>[8x]LEQKLISEEDLRSDKFRIMVQFLQANQESFMNGICGIMALASAQMYSSFEFTCPCLPDYNYA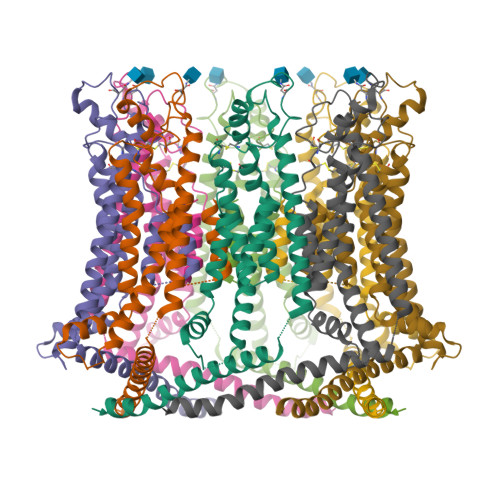YGIGILIVPPIWFFLLGYVMNNNISVLTEEWKRPVGKRSKDPAVLRYMFSSMTQRALIAPAVWIAVTLMDGKSFLCAFSPTADLSEFVNESYQSLSQKELLKIQAKIPCKDIFEEHEIISREAATRYIRCLSQACGWTFLMVITLVAFLVRAIRPCFTQAAFLKTKYWSHYIDTERKLFDETCKEHAKSFAKVCIQQYFESISGEIVSQLPQSPAKKGKGNKDEDGEKQKSDEERLLGIRKEGDMNKVLWNWHTCKPPLLLSKRTEEMNGHAHLDTHSLTDERHTKKKAVVYYSKV MALTOSYL-ALPHA (1,4)-(Z,3S,4S,5R,6R)-3,4,5-TRIHYDROXY-6-HYDROXYMETHYL-PIPERIDIN-2-ONE OXIME | C18 H32 N2 O15 | 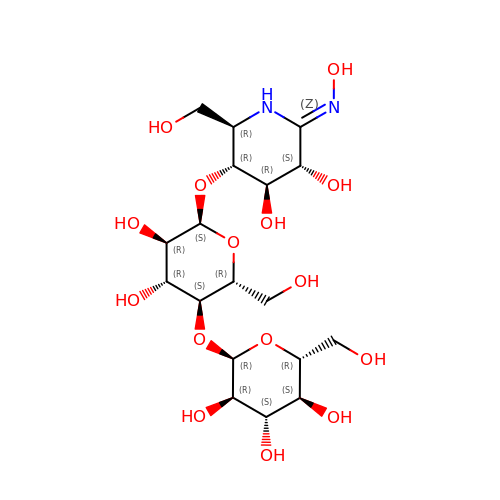AHRWQUNEPBVNOT-IVJVVCOPSA-N2,3-dihydro-1H-indene-2-carboxylic 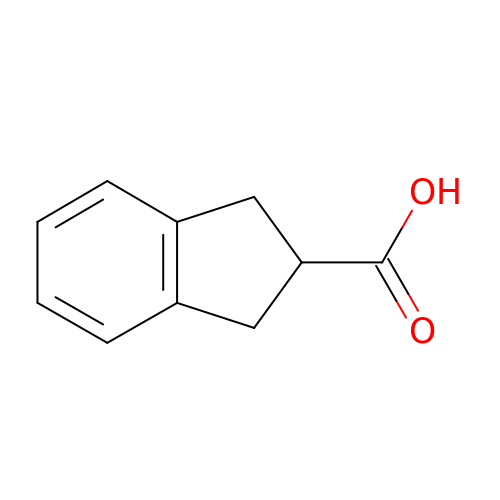acid | C10 H10 O2 | XUDCMQBOWOLYCF-UHFFFAOYSA-N> MKDILEKLEERRAQARLGGGEKRLEAQHKRGKLTARERIELLLDHGSFEEFDMFVQHRSTDFGMEKQKIPGDGVVTGWGTVNGRTVFLFSKDFTVFGGSSSEAHAAKIVKVQDMALKMRAPIIGIFDAGGARIQEGVAALGGHGEVFRRNVAASGVIPQISVIMGPCAGGDVYSPAMTDFIFMVRDTSYMFVTGPDVVKTVTNEVVTAEELGGAKVHTSKSSIADGSFENDVEAILQIRRLLDFL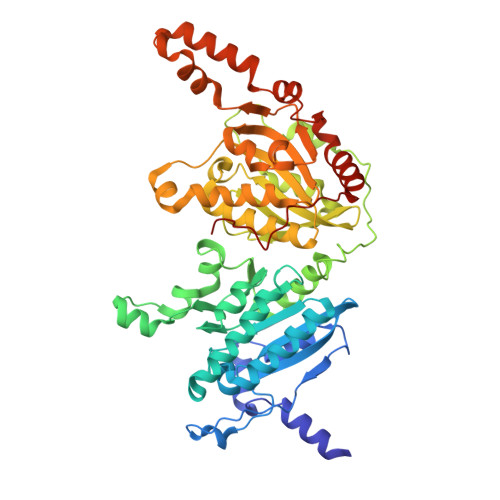PANNIEGVPEIESFDDVNRLDKSLDTLIPDNPNKPYDMGELIRRVVDEGDFFEIQAAYARNIITGFGRVEGRTVGFVANQPLVLAGVLDSDASRKAARFVRFCNAFSIPIVTFVDVPGFLPGTAQEYGGLIKHGAKLLFAYSQATVPLVTIITRKAFGGAYIVMASKHVGADLNYAWPTAQIAVMGAKGAVEIIFRAEIGDADKVAERTKEYEDRFLSPFVAAERGYIDEVIMPHSTRKRIARALGMLRTKEMEQPRKKHDNIPL>AEKPKAHYFNARGRMESTRWLLAAAGVEFEEKFIKSAEDLDKLRNDGYLMFQQVPMVEIDGMKLVQTRAILNYIASKYNLYGKDIKERALIDMYIEGIADLGEMILLLPVCPPEEKDAKLALIKEKIKNRYFPAFEKVLKSHGQDYLVGNKLSRADIHLVELLYYVEELDSSLISSFPLLKALKTRISNLPTVKKFLQPGSPRKP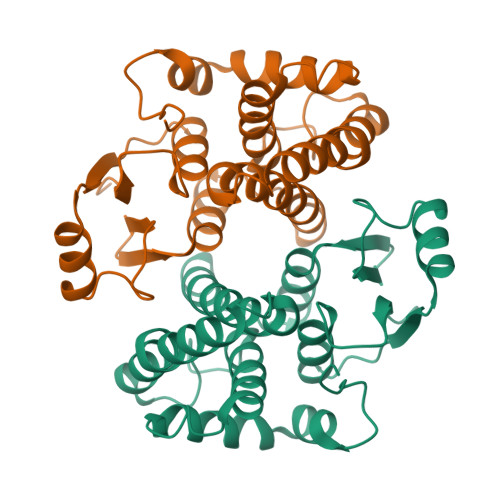PMDEKSLEEARKIFRF[2x]> GSPPEIKPFYFSSSVQEGQREQVICSAITGDLPLLFSWKKDGLIVENFKDITLVTNDLFSVLVISSIKPEHIGNYTCNLENPFGSDVHTAALTMKVPELS

Recently, a shortened Dscam (sDscam) gene family with tandemly arrayed 5′ cassettes in Chelicerata species has been identified, which encodes ∼50–100 isoforms. Chelicerata sDscams could be classified into two subfamilies, sDscamα and sDscamβ, containing one and two variable Ig domains, respectively. Crystal structures and cell aggregation assays demonstrated that both α and β subfamilies of sDscam used Ig1 for the isoform-specific trans recognition in a hand-in-hand manner. Furthermore, the cis interactions were established by the three FNIII domains of sDscam, which assemble into a cross fold with a kink between FNIII2 and FNIII3.

To elucidate the molecular details of trans interactions of sDscam, we determined the crystal structures of Ig1 from Mesobuthus martensii sDscam isoforms α1, α7, and β6v2. We also determined the crystal structures of sDscam Ig1 from another chelicerate species Limulus polyphemus (isoforms α7 and β3v7) to provide insights into the conservation of sDscam trans recognition within Chelicerata. These crystal structures of Ig fragments were determined at 1.3–3.1 Å resolutions. The crystal structures of sDscam Ig1 from both M. martensii and L. polyphemus revealed a common assembly of antiparallel homodimer for both α and β subfamilies of sDscam. More interestingly, in some Ig1 crystal structures (M. martensii α1, α7, and L. polyphemus α7), the two protomers within a homodimer were related via a 2-fold symmetry axis, namely, these two protomers had identical conformations. This implied that the homophilic trans interactions of Ig1 were also symmetry-related. Similarly, sDscam Ig1 also employs the ABED face to form an antiparallel homodimer. However, among the seven Ig1 structures reported here, the complementary electrostatic potential surface pattern (negative in one end, neutral in the middle, and positive in the other end) has been only observed in the three β isoforms, but not in any one of the four α isoforms. Structural analysis showed that B and E strands constituted the core of ABED face and dominated the trans homophilic interactions of sDscam Ig1. The residue preceding the conserved B-strand cystine always interacts with its counterpart of the other protomer.>[12x]SAEHVLTMLNEHEVKFVDLRFTDTKGKEQHVTIPAHQVNAEFFEEGKMFDGSSIGGWKGINESDMVLMPDASTAVIDPFFADSTLIIRCDILEPGTLQGYDRDPRSIAKRAEDYLRATGIADTVLFGPEPEFFLFDDIRFGASISGSHVAIDDIEGAWNSSTKYEGGNKGHRPGVKGGYFPVPPVDSAQDIRSEMCLVMEQMGLVVEAHHHE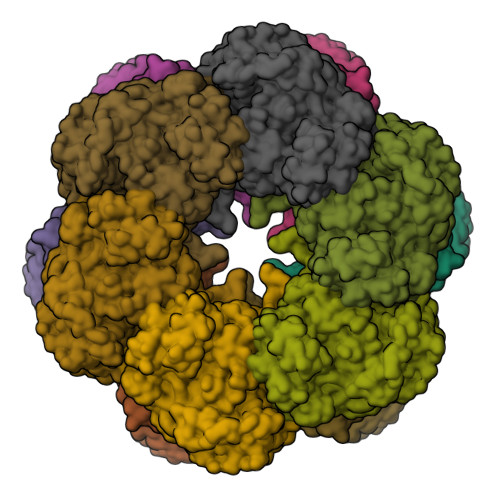VATAGQNEVATRFNTMTKKADEIQIYKYVVHNVAHRFGKTATFMPKPMFGDNGSGMHCHMSLAKNGTNLFSGDKYAGLSEQALYYIGGVIKHAKAINALANPTTNSYKRLVPGYEAPVMLAYSARNRSASIRIPVVASPKARRIEVRFPDPAANPYLCFAALLMAGLDGIKNKIHPGEPMDKNLYDLPPEEAKEIPQVAGSLEEALNALDLDREFLKAGGVFTDEAIDAYIALRREEDDRVRMTPHPVEFELYYSV>KSPAGFAEKYIIESIWNGRFPPGSILPAERELSELIGVTRTTLREVL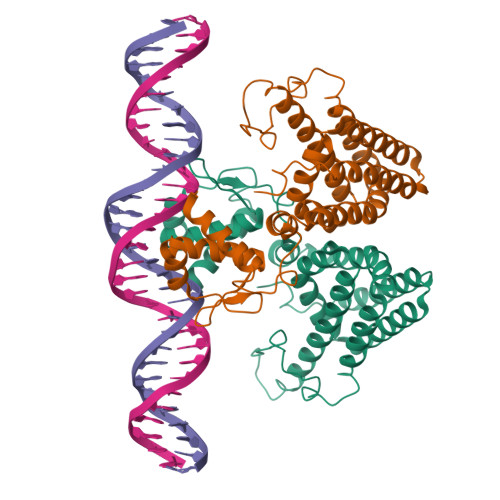QRLARDGWLTIQHGKPTKVNQFMETSGLHILDTLMTLDAENATSIVEDLLAARTNISPIFMRYAFKLNKESAERIMINVIESCEALVNAPSWDAFIAASPYAEKIQQHVKEDSEKDELKRQEILIAKTFNFYDYMLFQRLAFHSGNQIYGLIFNGLKKLYDRVGSYYFSNPQARELAMEFYRQLLAVCQSGEREHLPQVIRQYGIASGHIWNQMKMTLPSNFTED[4x]> MAEKEEAIFRSAEMALVQFYIPQEISRDSAYTLGQLGLVQFRDLNSKVRAFQRTFVNEIRRLDNVERQYRYFYSLLKKHDIKLYEGDTDKYLDGSGELYVPPSGSVIDDYVRNASYLEERLIQMEDATDQIEVQKNDLEQYRFILQSGDEFFLKGDNTDSTSYMDEDMIDANGENIAAAIGASVNYVTGVIARDKVATLEQILWRVLRGNLFFKTVEIEQPVYDVKTREYKHKNAFIVFSHGDLIIKRIRKIAESLDANLYDVDSSNEGRSQQLAKVNKNLSDLYTVLKTTSTTLESELYAIAKELDSWFQDVTREKAIFEILNKSNYDTNRKILIAEGWIPRDELATLQARLGEMIARLGIDVPSIIQVLDTNHTPPTFHRTNKFTAGFQSICDCYGIAQYREINAGLPTIVTFPFMFAIMFGDMGHGFLMTLAALSLVLNEKKINKMKRGEIFDMAFTGRYIILLMGVFSMYTGFLYNDIFSKTMTIFKSGWKW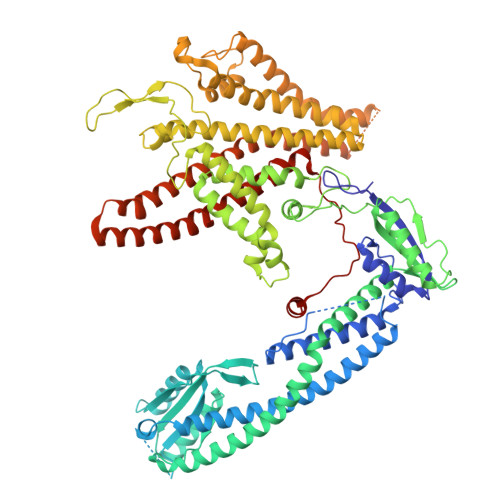PDHWKKGESITATSVGTYPIGLDWAWHGTENALLFSNSYKMKLSILMGFIHMTYSYFFSLANHLYFNSMIDIIGNFIPGLLFMQGIFGYLSVCIVYKWAVDWVKDGKPAPGLLNMLINMFLSPGTIDDELYPHQAKVQVFLLLMALVCIPWLLLVKPLHFKFTHKKKSHEPLPSTEADASSEDLEAQQLISAMDADDAEEEEVGSGSHGEDFGDIMIHQVIHTIEFCLNCVSHTASYLRLWALSLAHAQLSSVLWTMTIQIAFGFRGFVGVFMTVALFAMWFALTCAVLVLMEGTSAMLHSLRLHWVESMSKFFVGEGLPYEPFAFEYKDMEVAVASASSSASS The prototypical systems used to study sequential RNA assembly are group II introns, another class of highly-conserved self-splicing ribozymes of biomedical and bioengineering relevance. Group II introns are validated drug targets for antifungal antibiotics, potentially powerful vectors for genetic engineering, and the evolutionary ancestors of the catalytic RNA core of the eukaryotic spliceosome. Integrating single-particle electron cryomicroscopy (cryo-EM), image processing, in solution small-angle X-ray scattering (SAXS), EM-driven molecular dynamics (MD) simulations, structure-based mutagenesis, and enzymatic assays, we have visualized the sequential multidomain assembly of a self-splicing ribozyme of biomedical and bioengineering significance. Our work reveals a distinct dynamic interplay of helical subdomains in the ribozyme’s 5’-terminal scaffold, which acts as a gate to control the docking of 3’-terminal domains.

All these assembly intermediates are catalytically inactive as they lack the active site residues contributed by D521. F Density of the “fully open” state of D1-4 at 6.67 Å resolution. The other conformation, hereafter referred to as the “fully open” state, displays an even larger separation between D1c and i1-i2, a weak density for the ‘peripheral D1c’ motif, and disordered Z-anchor and θ nucleotides, which engage in tertiary contacts between D1 and D2. D3 only docks onto D1 in the D1-4 constructs, where however, D4 remains flexible and does not establish tertiary interactions with the rest of the molecule. In line with these chemical probing data, here we show that θ-θ’ is not stably formed in the “open” conformations of D1-2, D1-3, and D1-4.

> GUUAUGUGUGCCCGGCAUGGGUGCAGUCUAUAGGGUGAGAGUCCCGAACUGUGAAGGCAGAAGUAACAGUUAGCCUAACGCAAGGGUGUCCGUGGCGACAUGGAAUCUGAAGGAAGCGGACGGCAAACCUUCGGUCUGAGGAACACGAACUUCAUAUGAGGCUAGGUAUCAAUGGAUGAGUUUGCAUAACAAAACAAAGUCCUUUCUGCCAAAGUUGGUACAGAGUAAAUGAAGCAGAUUGAUGAAGGGAAAGACUGCAUUCUUACCCGGGGAGGUCUGGAAACAGAAGUCAGC> GSQIPASEQETLVRPK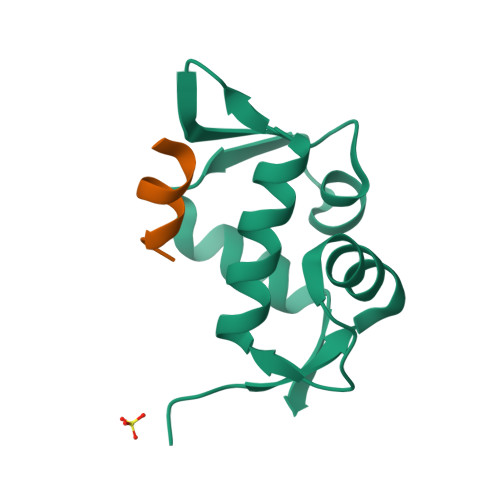PLLLKLLKSVGAQKDTYTMKEVLFYLGQYIMTKRLYDEKQQHIVYCSNDLLGDLFGVPSFSVKEHRKIYTMIYRNLVVVNQQESSDSGTSVSEN;> RFMDYWEGL>[2x]MTADGPRELLQLRAAVRHRPQDFVAWLMLADAELGMGDTTAGEMAVQRGLALHPGHPEAVARLGRVRWTQQRHAEAAVLLQQASDAAPEHPGIALWLGHALEDAGQAEAAAAAYTRAHQLLPEEPYITAQLLNWRRRLCDWRALDVLSAQVRAAVAQGVGAVEPFAFLSEDASAAEQLACARTRAQAIAASVRPLAPTRVRSKGPLRVGFVSNGFGAHPTGLLTVALFEALQRRQPDLQMHLFATSGDDGSTLRTRLAQASTLHDVTALGHLATAKHIRHHGIDLLFDLRGWGGGGRPEVFALRPAPVQVNWLAYPGTSGA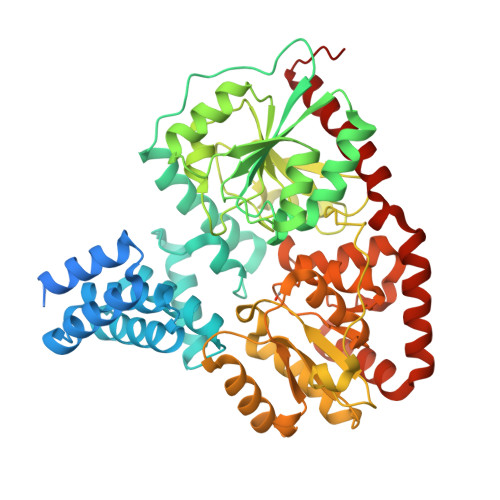PWMDYVLGDAFALPPALEPFYSEHVLRLQGAFQPSDTSRVVAEPPSRTQCGLPEQGVVLCCFNNSYKLNPQSMARMLAVLREVPDSVLWLLSGPGEADARLRAFAHAQGVDAQRLVFMPKLPHPQYLARYRHADLFLDTHPYNAHTTASDALWTGCPVLTTPGETFAARVAGSLNHHLGLDEMNVADDAAFVAKAVALASDPAALTALHARVDVLRRASGVFHMDGFADDFGALLQALARRHGWLGI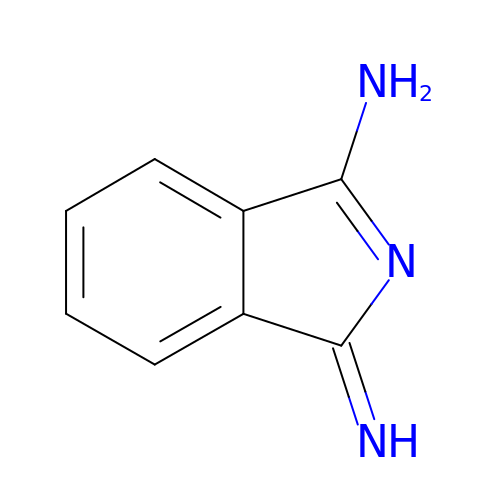(1Z)-1-imino-1H-isoindol-3-amine | C8 H7 N3 | RZVCEPSDYHAHLX-UHFFFAOYSA-N N-[(1R)-1-carboxy-3-phenylpropyl]-L-leucyl-L-tryptophan 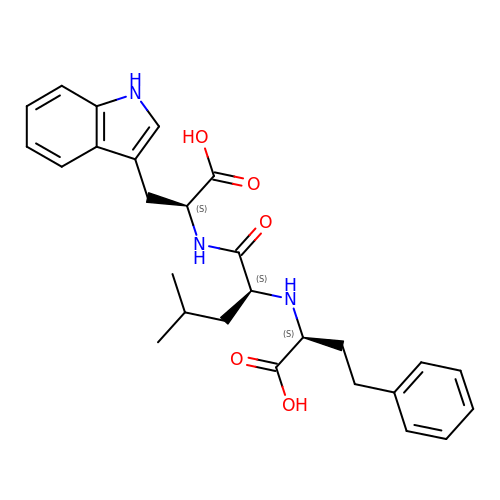| C27 H33 N3 O5 | PAPCSVADGJFRFM-HJOGWXRNSA-N>[6x]MPLISSSIPNLINGVSQQPAALRLASQAEEVINCMPSPVEGLKKRPPMQHIKKLFAGSAGTGRPFTHIVDRDGVIRYLIFIQDNAIKVFDLDGNAQTVSTPNGTSYLNITGEPSSTFRVASIADFTFIVNREKTVAMDTTNKSYNWGTKSMVFIKSADFSTTYRVKLN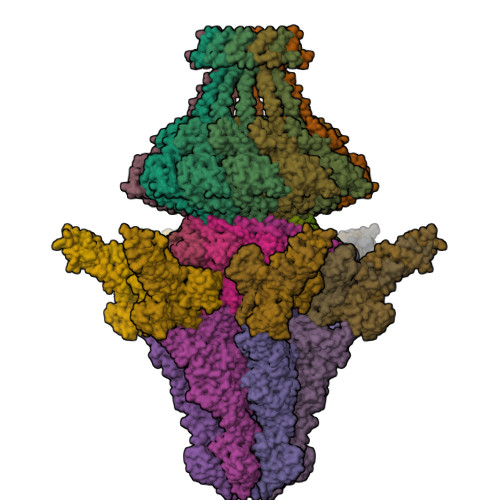GTEKSVTTGNSSGSAPDTVTIASDLATQLNTISGFTVTSTDYIIRITKDDGGDYTLESSDTKTADATSAIKGTVDSITDLPTIAEHNFTVRIQGSATTAFDDYFVKFEATAGSGFGPGVWRETVAPNIDHLLDKSTMPHTLVRNANGTFTFAQFNYTGRVAGDTTTAPNPTFVGSKIKNINLFRNRLVFLADENVILSAADSFERFFPETVQTLLDSDPIDISSGGTSVNFLNSSLAFANTLLLFSLHGQFRLDTGSTSVGTALTPKTATITAITTFDIVDAIDPIGVGRTVYFGIPKGDFSGLREYFLPDASGPIPLSEEVTSSVPRFVPGNLISMSPSVSEEVITMISKDQPRRVYIYKFFFDDDQKLQSSWSYWEVAANKTLLGGNVLDSDLYTCVEYSDGVYLEKTQLRPETVDSGTEFEILLDRKTTEAACSTSLINSGALGVQTVITLPYPMSGTGTMAVVGRFASNNTIAHGQVIKATAETLTGGASGNGTMTVPGDLSSAKFFVGEIYNMTYEFSTPYLKETPPGGGLAVLANPRLQLRTWSIVFDETSNFSMKITPGQRDELTYPFNGYKIGSGQFPIGTPSLATGRFRVPVMAQNIETKIVLFSDSPLPCRVQSAEWEGWYQERARRL;>MAARTSFLDAVNRVLQMLGEAPVNSLQGQFGLAKQAEVALNDVSRTIQTEGWSFNTDLEKKLERNSSNEIELSSNVSRVVVDNLEYPDIDVVQRGDKLYDRKNNRYTFDEDLIVDMTTILEWDLLPEHARQYITIKAGRQLQEAIIGSAELTKLNLTQEVEARSAFLEEETTKSEHSMLRGHLNRTSPVNTYIPSRTLER[12x];>MAFAQRIITSNSAGDQEFTFTFDYIKEEHIKVFVNFVEKAQGTGSNEFQVITNTTPKKISLNTGLSADNTRVEIRRVSSLSTPLVDFADGSTLTAADLDTAEKQSLFIDQELDDALKQGISIDTSTGVPTLNSQRLSNVSDPVNAQDAVTKAYLERSGSITSTQILNGTIVDADINASAAIAKSKLAALNIVNADVNASAAIAGSKLADASIAYTKIQNVSATNRILGRDSSGAGVIEEITPANLRTMINVEDGATADQSAAEIRTLVESASDSNVFTDADHTKLNAIEASADVTDATNVDAAGAVMNSDTSTAAMQFVIDEDTFGSNLDTKVPTQQSVKAYITATSQPLDSELSQLAGMQSGTASKLADSTALTADIADLNQLDGMAKETSITNSNTKFPTSAAVVNFVANQIAPVGGLEVIADEDSFPATQPVSGVVISISNADGLVINNAGEASNARTVGSGSDNVTIKNFPASLRNQTLAPNLGLLVSSTGASQEYNYHKLLAKETDVLQLSDDINDFNNRYRVENTLPAANDSSNHDGDLVYAKEEKKIYVYSGDYNGTPVGSFGEVQSIGNFFISTLSPAFNGSLQDFTITNAPSNAQQIILSINGVIQKPNSGTSTPSEGFALSGSTIKLAAAPPSGADYFAIVLGSTVNIGTPSNNTVTSSILQNGSVIEAKLGSGAVTRTKLNLVSTSSAPGLEVKGDGSSDGYLQLNCSQNSHGIKLKSPPHSAGQSYTLTFPSNIVSGQFLTTDANGNLSWAAVVTDLVNDTSPQLGGNLDCNDKNILLNDSSGSANNRIRLGASQDFALFHNGTINIIEAVSGDLHLRLNGSEEGIIVKQNGAVELYYDNSKKFHTSSVGATVTGNLFLSGGYINLNDNYSYGMGSGNRAQLYHSGNHQYLLNTVGNMYFQPKSGENGIVIIPDDAVELYHNNVKRLETTSGGVTVSGSVTATGHLFVGANTHYLYFTSTAGYSPRIGNADGGTGVNMTFHTNNTMRMMLQNDGHLRPASNNTYDLGTSSDRWRNVYTNDLNLSNEGGANDVDGTWGSYTIQEGAEDLFLINKRTSKKYKFNLTEVS[18x];>MKTRLTNNVDRQSALYGSSGGTAAQRYEQLRVDRNSPLKRARDCSKVTIPGLIEDENYGDAGRLDTPYQSSGARGVGHMTSKLAVTLFPTNEHFFKLEIDSLAILASDQNPEMITEFDSALVKVEQAVMRMFETIGGRAAMHEALKHLLVGGNVLLYVSDEGIKVIHLDSYVLCRDPMGNVTEIVVEEEIFKDALPEEYLDEEDDDDDDMGKKMVKIYTCIKFMDDQCHWYQEIKGKEVPGTHGKCAADVAPWIALRQDRVDSEMYGRSYVEQYYGDLLALENLYKAILEASASLSKVLFLCNPNGTTRPRTLSQASNGSIVQGNAADVTVLQAAGKSQDLQIANQTIERIENRLAFAFMLNTAIQRPGERVTAEEIRYMAQELDAGISGLYSILSRELQLPLVRRLIHILRRKRKLPDFPRSEVTGEPLIKEKAVTGIEAIGRGDDRNKLIDFITTANQALGPQAMTQFLNVEEALRRLAASGSIDTTNLVKTKAQLQQEAAAQAEAEQQAQQQQLLETGIKSPAMAQAVKNFQGADPERAAQALSAITSETGGIDADQLTEAV[12x]> MSEAGNVASGLGLPGEVSQWSLKRYGRFMLLDNVGSPGPSSEAAAAGSSTWKVFESSEESGS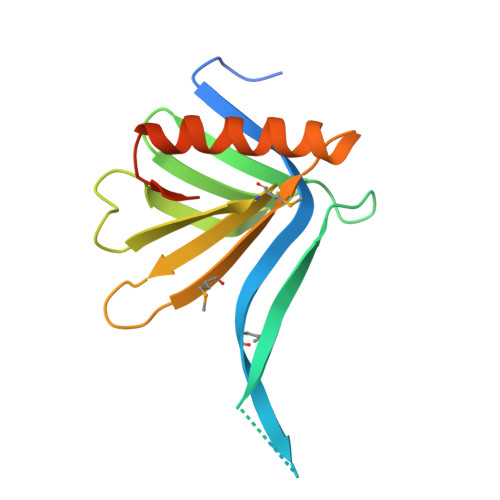LVLTIVVSGHFFISQGQTLLEGFSLIGSKNWLKIVRRMDCLLFGTTIKNKSRMFRVQFSGESKEEALERCCGCVQTLAQYVTVQEPDSTTQELQQS>[2x]NVADGF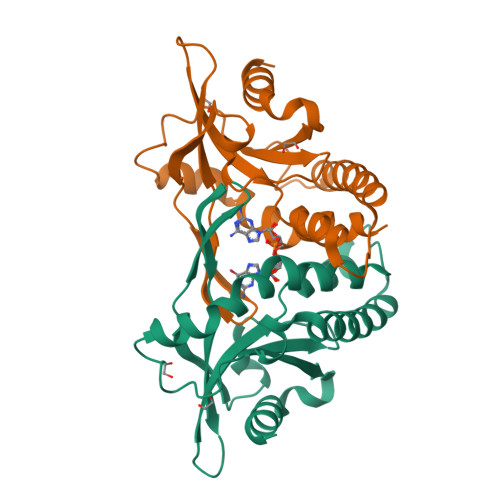AWNYYFGYLKLVLPRLEAQIAKSSEFRYKITKKKLYILVPKTCYVYDNIADADPRVTWAGDLTPCKINRGGIKERIYKQAVYRVAMTDKHEYFFILEYASNLMSLYDMSLHEDAPLSRQERDDQVVLFIRKLREILEGCKECRGKCEIVPISGDEKSKIADVLVAIHNATQVESDEADL>SASVRIREAKEGDCGDILRLIRELAEFEKLSDQVKISEEALRADGFGDNPFYHCLVAEILPAPGKLLGPCVVGYGIYYFIYSTWKGRTIYLEDIYVMPEYRGQGIGSKIIKKVAEVALDKGCSQFRLAVLDWNQRAMDLYKALGAQDLTE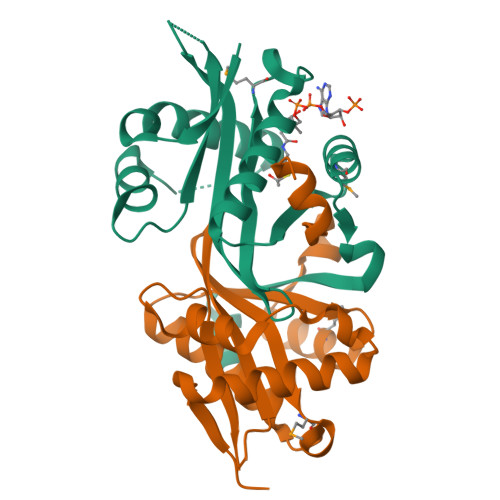AEGWHFFCFQGEATRKLAGK[2x]>[2x]MKVFNRPILFDIVSRGSPDGLEGLLSFLLTHKKRLTDEEFREPSTGKTCLPKALLNLSAGRNDTIPILLDIAEKTGNMREFINSPFRDVYYRGQTALHIAIERRCKHYVELLVEKGADVHAQARGRFFQPKDEGGYFYFGELPLSLAAC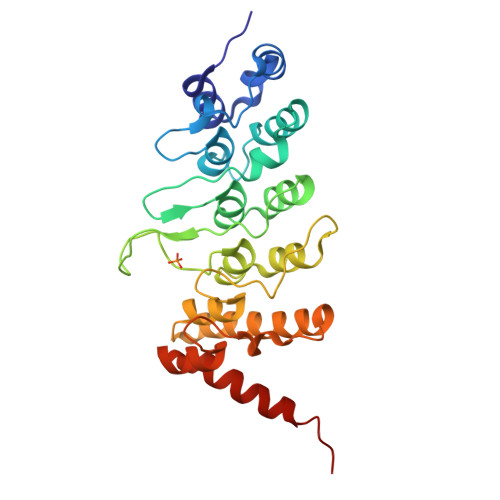TNQPHIVHYLTENGHKQADLRRQDSRGNTVLHALVAIADNTRENTKFVTKMYDLLLIKCAKLFPDTNLEALLNNDGLSPLMMAAKTGKIGIFQHIIRREIADAAAHHHHHH Parkinson’s-disease-associated LRRK2 kinase phosphorylates Rab8a and Rab10 to subvert their membrane trafficking functions in the formation of primary cilia. Rab8a is phosphorylated at a threonine (pT72) and subsequently binds to a phosphospecific effector (RILPL2) via its C-terminal RH2 domain. The C-terminal RH2 domain of RILPL2 encodes a Rab-binding domain (RBD) that adopts a parallel α-helical coiled-coil structure. Here, we show that recognition of pT72 involves a dual arginine motif involving R130 and R132 from the RH2 domain of RILPL2.

Here, we have determined the structure of pRab8a in a complex with an extended RBD of RILPL2 (117–165; abbreviated as RL2117) at 1.9-Å resolution. The structure includes residues preceding the X-cap that were not mapped in our previous work. The structure of GTP-bound pRab8(Q67L) in complex with RL2117 forms crystals with one molecule of pRab8a and one molecule of RILPL2 as the repeating unit. The biological heterotetramer is generated by a twofold crystallographic axis down the length of the central parallel α-helical dimer of RL2117. Although the RBD of the complex begins at 117, residues 117–125 are disordered. The model contains residues 126–161 of RILPL2 and resembles closely the minimal RBD (129–161) of the previous structure (pRab8a:RILP129 complex). The complex with the extended RBD (RL2117) has two well-ordered stacked arginines in which R130 appears to stabilize the conformation of R132, which directly forms a salt bridge to the pT72R8. Strikingly, the newly determined structure of pRab8a:RL2117 reveals an ordered R130 side chain that forms strong stacking interactions with the guanidino group of R130. As a measure of the close contacts, the distance between R130(Nε) and R132(NH2) is 3.4 Å. In contrast to the other complexes, pRab8a:RILP117 forms a symmetric twofold axis down the length of the coiled coil.

> GSHMAKTYDYLFKLLLIGDSGVGKTCVLFRFSEDAFNSTFISTIGIDFKIRTIELDGKRIKLQIWDTAGLERFRTITTAYYRGAMGIMLVYDITNEKSFDNIRNWIRNIEEHASADVEKMILGNKCDVNDKRQVSKERGEKLALDYGIKFMETSAKANINVENAFFTLARDIKAKMDKKLEGNS;> GSHMGPNKMVVDLTDPNRPRFTLQELRDVLQERNKLKSQLLVVQEELQCYKSG>[3x]SSKLSIISWNVDGLDTNNLSDRARGLCSYLALYTPDVVFLQELIPAYVQYLKKRAVSYLFFEGSDDGYFTGIMLRKSRVKFLESEIICFPTTQ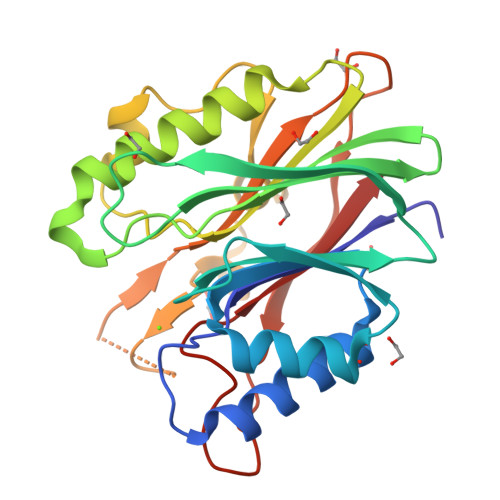MMRNLLIAQVTFSGQKLYLMTSHLESTRNQSQERTKQLRVVLQKIKEAPEDAIVIFAGDTNLRDAEVANVGGLPAGVCDVWEQLGKQEHCRYTWDTQANSNLGITAACKLRFDRIFLRSAKTAPPVTPDHMALIGMEKLDCGRYTSDHWGIYCTFNT>[2x]MASGSCQGCEEDEETLKKLIVRLNNVQEGKQIETLVQILEDLLVFTYSERASKLFQGKNIHVPLLIVLDSYMRVASVQQVGWSLLCKLIEVCPGTMQSLMGPQDVGND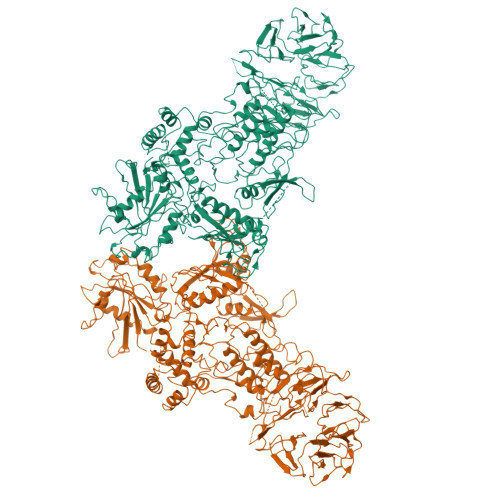WEVLGVHQLILKMLTVHNASVNLSVIGLKTLDLLLTSGKITLLILDEESDIFMLIFDAMHSFPANDEVQKLGCKALHVLFERVSEEQLTEFVENKDYMILLSALTNFKDEEEIVLHVLHCLHSLAIPCNNVEVLMSGNVRCYNIVVEAMKAFPMSERIQEVSCCLLHRLTLGNFFNILVLNEVHEFVVKAVQQYPENAALQISALSCLALLTETIFLNQDLEEKNENQENDDEGEEDKLFWLEACYKALTWHRKNKHVQEAACWALNNLLMYQNSLHEKIGDEDGHFPAHREVMLSMLMHSSSKEVFQASANALSTLLEQNVNFRKILLSKGIHLNVLELMQKHIHSPEVAESGCKMLNHLFEGSNTSLDIMAAVVPKILTVMKRHETSLPVQLEALRAILHFIVPGMPEESREDTEFHHKLNMVKKQCFKNDIHKLVLAALNRFIGNPGIQKCGLKVISSIVHFPDALEMLSLEGAMDSVLHTLQMYPDDQEIQCLGLSLIGYLITKKNVFIGTGHLLAKILVSSLYRFKDVAEIQTKGFQTILAILKLSASFSKLLVHHSFDLVIFHQMSSNIMEQKDQQFLNLCCKCFAKVAMDDYLKNVMLERACDQNNSIMVECLLLLGADANQAKEGSSLICQVCEKESSPKLVELLLNSGSREQDVRKALTISIGKGDSQIISLLLRRLALDVANNSICLGGFCIGKVEPSWLGPLFPDKTSNLRKQTNIASTLARMVIRYQMKSAVEEGTASGSDGNFSEDVLSKFDEWTFIPDSSMDSVFAQSDDLDSEGSEGSFLVKKKSNSISVGEFYRDAVLQRCSPNLQRHSNSLGPIFDHEDLLKRKRKILSSDDSLRSSKLQSHMRHSDSISSLASEREYITSLDLSANELRDIDALSQKCCISVHLEHLEKLELHQNALTSFPQQLCETLKSLTHLDLHSNKFTSFPSYLLKMSCIANLDVSRNDIGPSVVLDPTVKCPTLKQFNLSYNQLSFVPENLTDVVEKLEQLILEGNKISGICSPLRLKELKILNLSKNHISSLSENFLEACPKVESFSARMNFLAAMPFLPPSMTILKLSQNKFSCIPEAILNLPHLRSLDMSSNDIQYLPGPAHWKSLNLRELLFSHNQISILDLSEKAYLWSRVEKLHLSHNKLKEIPPEIGCLENLTSLDVSYNLELRSFPNEMGKLSKIWDLPLDELHLNFDFKHIGCKAKDIIRFLQQRLKKAVPYNRMKLMIVGNTGSGKTTLLQQLMKTKKSDLGMQSATVGIDVKDWPIQIRDKRKRDLVLNVWDFAGREEFYSTHPHFMTQRALYLAVYDLSKGQAEVDAMKPWLFNIKARASSSPVILVGTHLDVSDEKQRKACMSKITKELLNKRGFPAIRDYHFVNATEESDALAKLRKTIINESLNFKIRDQLVVGQLIPDCYVELEKIILSERKNVPIEFPVIDRKRLLQLVRENQLQLDENELPHAVHFLNESGVLLHFQDPALQLSDLYFVEPKWLCKIMAQILTVKVEGCPKHPKGIISRRDVEKFLSKKRKFPKNYMSQYFKLLEKFQIALPIGEEYLLVPSSLSDHRPVIELPHCENSEIIIRLYEMPYFPMGFWSRLINRLLEISPYMLSGRERALRPNRMYWRQGIYLNWSPEAYCLVGSEVLDNHPESFLKITVPSCRKGCILLGQVVDHIDSLMEEWFPGLLEIDICGEGETLLKKWALYSFNDGEEHQKILLDDLMKKAEEGDLLVNPDQPRLTIPISQIAPDLILADLPRNIMLNNDELEFEQAPEFLLGDGSFGSVYRAAYEGEEVAVKIFNKHTSLRLLRQELVVLCHLHHPSLISLLAAGIRPRMLVMELASKGSLDRLLQQDKASLTRTLQHRIALHVADGLRYLHSAMIIYRDLKPHNVLLFTLYPNAAIIAKIADYGTAQYCCRMGIKTSEGTPGFRAPEVARGNVIYNQQADVYSFGLLLYDILTTGGRIVEGLKFPNEFDELEIQGKLPDPVKEYGCAPWPMVEKLIKQCLKENPQERPTSAQVFDILNSAELVCLTRRILLPKNVIVECMVATHHNSRNASIWLGCGHTDRGQLSFLDLNTEGYTSEEVADSRILCLALVHLPVEKESWIVSGTQSGTLLVINTEDGKKRHTLEKMTDSVTCLYCNSFSKQSKQKNFLLVGTADGKLAIFEDKTVKLKGAAPLKILNIGNVSTPLMCLSESTNSTERNVMWGGCGTKIFSFSNDFTIQKLIETRTSQLFSYAAFSDSNIITVVVDTALYIAKQNSPVVEVWDKKTEKLCGLIDCVHFLREVMVKENKESKHKMSYSGRVKTLCLQKNTALWIGTGGGHILLLDLSTRRLIRVIYNFCNSVRVMMTAQLGSLKNVMLVLGYNRKNTEGTQKQKEIQSCLTVWDINLPHEVQNLEKHIEVRKELAEKMRRTSVE One intriguing example is the African swine fever virus, which stands as the sole mammalian-infecting virus encoding a type II topoisomerase. The ORF P1192R encodes a functional Topo II (pP1192R) which is highly conserved across diverse ASFV isolates. Prior extensive structural and biochemical studies have elucidated key aspects of Topo II catalytic mechanisms. These structures have unveiled the inherent architecture of Topo II, which is characterized by two principal heart-shaped functional domains: the ATPase domain, responsible for ATP hydrolysis to fuel the molecular machinery, and the central domain, which interacts with the DNA duplex and contains a catalytic tyrosine residue that cleaves the DNA duplex. As a result, Topo II not only relaxes DNA supercoiling but also disentangles knots and catenates potentially detrimental to cellular function if left unresolved.

In parallel, the full-length pP1192R was mixed with 52 bp DNA oligonucleotides, Mg2+ and AMPPNP, which was subsequently plunged-frozen on an amorphous alloy film (R1.2/1.3, Au, 300 mesh) at the same concentration. During the course of cryo-EM image processing from the dataset, we determined three distinct full-length pP1192R structures, each characterized by a unique orientation of the ATPase domain in relation to the central domain: pP1192RF1, pP1192RF2, and pP1192RF3. The atomic model of pP1192R-DNA complex encompasses a homodimer of the GHKL, Transducer, TOPRIM, WHD, Tower and Coiled-Coil subdomains, alongside a curving DNA duplex. A pliable short linker (aa 410-420) interconnects these two domains, accounting for the wobbling of the ATPase domain. Collaboratively, the TOPRIM, WHD and Tower subdomains constitute a positively charged DNA binding groove that accommodates a DNA duplex. The DNA duplex engages in an extensive interaction with the DNA binding groove of pP1192R. Meanwhile, the Tower subdomain presents an additional β-hairpin, referred to as wing-2 (847-860). This wing-2 motif adeptly intercalates itself amidst the base stacks of the bound DNA, facilitating a global DNA bending of ~150° and a localized DNA conformational transition from the B-form to the A-form. However, the ATPase domain retains a flexible conformation, which likely correlates with the energy transfer dynamics intrinsic to the DNA cleavage/stand passage process. In the full-length structures, a continuous wobbling characterizes the ATPase domain, suggesting a plausible correlation between the rotation of the ATPase domain and the oscillatory behavior of the central domain9.

>[2x]EFATMEAFEISDFKEHAKKKSMWAGALNKVTISGLMGVFTEDEDLMALPIHRDHCPALLKIFDEIIVNATDHERACHNKTKKVTYIKISFDKGVFSCENDGPGIPIAKHEQASLIAKRDVYVPEVASCHFLAGTNINKAKDCIKGGTNGVGLKLAMVHSQWAILTTADGAQKYVQHINQRLDIIEPPTITPSREMFTRIELMPVYQELGYAEPLSETEQADLSAWIYLRACQCAAYVGKGTTIYYNDKPCRTGSVMALAKMYTLLSAPNSTIHTATIKADAKPYSLHPLQVAAVVSPKFKKFEHVSVINGVNCVKGEHVTFLKKTINEMVVKKFQQTIKDKNRKTTLRDSCSNIFIVIVGSIPGIEWTGQRKDELSIAENVFKTHYSIPSSFLTSMTKSIVDILLQSISKKDNHKQVDVDKYTRARNAGGKRAQDCMLLAAEGDSALSLLRTGLTLGKSNPSGPSFDFCGMISLGGVIMNACKKVTNITTDSGETIMVRNEQLTNNKVLQGIVQVLGLDFNCHYKTQEERAKLRYGCIVACVDQDLDGCGKILGLLLAYFHLFWPQLIIHGFVKRLLTPLIRVYEKGKTMPVEFYYEQEFDAWAKKQTSLANHTVKYYKGLAAHDTHEVKSMFKHFDNMVYTFTLDDSAKELFHIYFGGESELRKRELCTGVVPLTETQTQSIHSVRRIPCSLHLQVDTKAYKLDAIERQIPNFLDGMTRARRKILAGGVKCFASNNRERKVFQFGGYVADHMFYHHGDMSLNTSIIKAAQYYPGSSHLYPVFIGIGSFGSRHLGGKDAGSPRYISVQLASEFIKTMFPAEDSWLLPYVFEDGQRAEPEYYVPVLPLAIMEYGANPSEGWKYTTWARQLEDILALVRAYVDKDNPKHELLHYAIKHKITILPLRPSNYNFKGHLKRFGQYYYSYGTYVISEQRNIITITELPLRVPTVAYIESIKKSSNRMTFIEEIIDYSSSETIEILVKLKPNSLNRIVEEFKETEEQDSIENFLRLRNCLHSHLNFVKPKGGIIEFNTYYEILYAWLPYRRELYQKRLMREHAVLKLRIIMETAIVRYINESAELNLSHYEDEKEASRILSEHGFPPLNHTLIISPEFASIEELNQKALQGCYTYILSLQARELLIAAKTRRVEKIKKMQARLDKVEQLLQESPFPGASVWLEEIDAVEKAIIKGRNTQWKFHENLYFQGHHHHHHHH Pregnancy-Associated Plasma Protein A isoforms, PAPP-A and PAPP-A2, are metalloproteases that cleave insulin-like growth factor binding proteins (IGFBPs) to modulate insulin-like growth factor signaling. PAPP-A2 shares 46% sequence conservation with PAPP-A (with mature numbering for both proteins used in the text). Both PAPP-A2 and PAPP-A contain an N-terminal Laminin-G (LG) domain and a catalytic metalloprotease (MP) domain that itself contains two Lin12-Notch repeats (LNR1 and LNR2). PAPP-A specifically cleaves IGFBP2, IGFBP4, and IGFBP-5, and its cleavage of IGFBP2 and IGFBP4 is IGF-dependent, while PAPP-A2 cleaves IGFBP3 and IGFBP5 in an IGF independent manner.

Here, we present the single-particle cryo-EM structure of the monomeric, N-terminal LG, MP, and the M1 domains (with the exception of LNR1/2) of human PAPP-A2 to 3.13 Å resolution. However, no IGFBP5 density was observed in the structure, suggesting substrate dissociation during the preparation process, and thus we treated the structure as apo PAPP-A2. The structure was reconstructed to 3.13 Å resolution, which allowed us to build a model corresponding to residues 25-926, except for residues 373 – 420 in the LNR1 and LNR2 regions that featured ambiguous map density. No density was present for the M2 domain, CCP1-5 domains, or the LNR3 domain, suggesting that these regions are flexible. PAPP-A2 is glycosylated and we observed clear density corresponding to stabilized glycans bound to residues N328 and N445 that we modeled as N-acetylglucosamine (yellow sticks). PAPP-A2 is a monomer by cryo-EM reconstruction. The active sites of PAPP-A and PAPP-A2 overlay with an RMSD of 0.35 Å. PAPP-A2 features a characteristic metzincin HEXXHXXGXXH motif21 where zinc is coordinated by H499, H503, and H509, and the catalytic E500 (mutated to Q in our structure) is 3.2 Å away from the histidine cluster (with map density shown in Supplementary Fig. 2h). Interestingly, we observed the catalytic water that is coordinated by zinc and hydrogen bonds to Y575. The observed PAPP-A2 domains align with the N-terminal domains of one monomer of the PAPP-ABP5 structure with a root mean squared deviation (RMSD) score of 2.0 Å. The A799V point mutation occurs in a region of the M1 domain that is over 26 Å away from the catalytic zinc as revealed by our cryo-EM structure.

> PPEESNQNGGEGSYREAETFNSQVGLPILYFSGRRERLLLRPEVLAEIPREAFTVEAWVKPEGGQNNPAIIAGVFDNCSHTVSDKGWALGIRSGKDKGKRDARFFFSLCTDRVKKATILISHSRYQPGTWTHVAATYDGRHMALYVDGTQVASSLDQSGPLNSPFMASCRSLLLGGDSSEDGHYFRGHLGTLVFWSTALPQSHFQHSSQHSSGEEEATDLVLTASFEPVNTEWVPFRDEKYPRLEVLQGFEPEPEILSPLQPPLCGQTVCDNVELISQYNGYWPLRGEKVIRYQVVNICDDEGLNPIVSEEQIRLQHEALNEAFSRYNISWQLSVHQVHNSTLRHRVVLVNCEPSKIGNDHCDPECEHPLTGYDGGDCRLQGRCYSWNRRDGLCHVECNNMLNDFDDGDCCDPQVADVRKTCFDPDSPKRAYMSVKELKEALQLNSTHFLNIYFASSVREDLAGAATWPWDKDAVTHLGGIVLSPAYYGMPGHTDTMIHQVGHVLGLYHVFKGVSERESCNDPCKETVPSMETGDLCADTAPTPKSELCREPEPTSDTCGFTRFPGAPFTNYMSYTDDNCTDNFTPNQVARMHCYLDLVYQQWTESRKPTPIPIPPMVIGQTNKSLTIHWLPPISGVVYDRASGSLCGACTEDGTFRQYVHTASSRRVCDSSGYWTPEEAVGPPDVDQPCEPSLQAWSPEVHLYHMNMTVPCPTEGCSLELLFQHPVQADTLTLWVTSFFMESSQVLFDTEILLENKESVHLGPLDTFCDIPLTIKLHVDGKVSGVKVYTFDERIEIDAALLTSQPHSPLCSGCRPVRYQVLRDPPFASGLPVVVTHSHRKFTDVEVTPGQMYQYQVLAEAGGELGEASPPLNHIHGAPYCGDGKVSERLGEECDDGDLVSGDGCSKVCELEEGFNCVGEPSLCYMYEGDGICEPFERKTSIVDCGIYTPKGYLDQWATRAYSSHEDKKKCPVSLVTGEPHSLICTSYHPDLPNHRPLTGWFPCVASENETQDDRSEQPEGSLKKEDEVWLKVCFNRPGEARAIFIFLTTDGLVPGEHQQPTVTLYLTDVRGSNHSLGTYGLSCQHNPLIINVTHHQNVLFHHTTSVLLNFSSPRVGISAVALRTSSRIGLSAPSNCISEDEGQNHQGQSCIHRPCGKQDSCPSLLLDHADVVNCTSIGPGLMKCAITCQRGFALQASSGQYIRPMQKEILLTCSSGHWDQNVSCLPVDCGVPDPSLVNYANFSCSEGTKFLKRCSISCVPPAKLQGLSPWLTCLEDGLWSLPEVYCKLECDAPPIILNANLLLPHCLQDNHDVGTICKYECKPGYYVAESAEGKVRNKLLKIQCLEGGIWEQGSCIPVVCEPPPPVFEGMYECTNGFSLDSQCVLNCNQEREKLPILCTKEGLWTQEFKLCENLQGECPPPPSELNSVEYKCEQGYGIGAVCSPLCVIPPSDPVMLPENITADTLEHWMEPVKVQSIVCTGRRQWHPDPVLVHCIQSCEPFQADGWCDTINNRAYCHYDGGDCCSSTLSSKKVIPFAADCDLDECTCRDPKAEENQTRTGGDYKDDDDK> GAERTIQLPKPDMNRAGLLMKALSERHSTREYASKALSNTDLSDLLWAANGINRSSEGKRTAPSAMNRQDIDIYVVLPQGTYLYD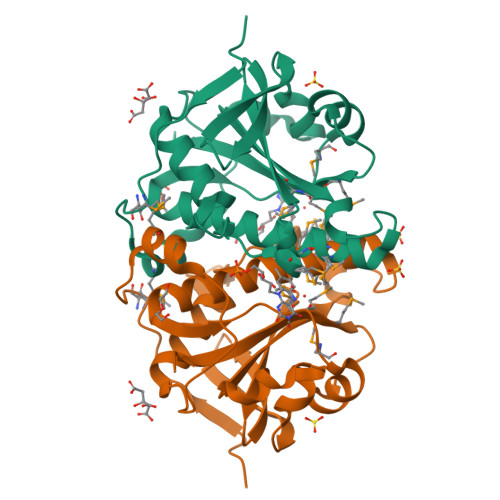AKGHKLNLISEGDHRSAVAGGQAFVNNAPVSLVLVSDLSKLGDAKSNHVQLMGAMDAGIVSQNISLFCSAARLATVPRASMDLVRLKAALKLKDTQMPMMNHPVGYFK(2S)-2-[3-(aminomethyl)benzyl]-3-[(R)-[(1R)-1-amino-3-phenylpropyl](hydroxy)phosphoryl]propanoic acid | C20 H27 N2 O4 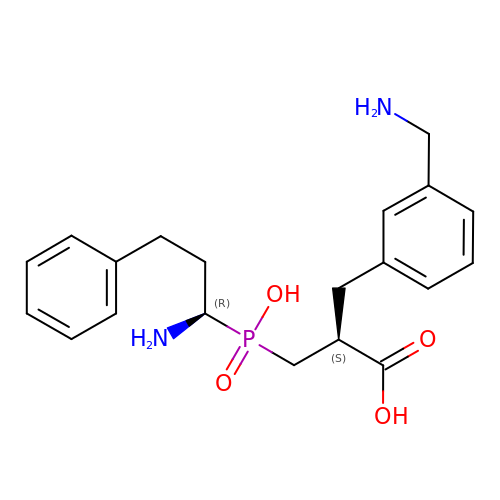P | OGZYJUYHRXGJNP-RTBURBONSA-N>[6x]GSPGISGGGGGILELIGDYSKAFLLQTVDGKHQDLKYISPETMVALLTGKFSNIVDKFVIVDCRYPYEYE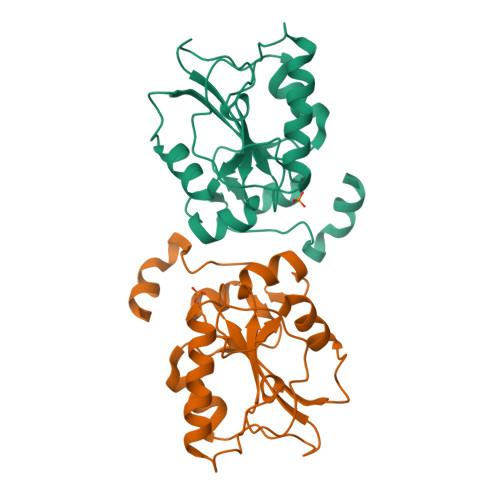GGHIKTAVNLPLERDAESFLLKSPIAPCSLDKRVILIFHCEFSSERGPRMCRFIRERDRAVNDYPSLYYPEMYILKGGYKEFFPQHPNFCEPQDYRPMNHEAFKDELKTFRLKTRSWAGERSRRELCSRLQDQ We previously demonstrated that MilA, a CMP hydroxymethylase in the mildiomycin biosynthetic gene cluster in Streptomyces rimofaciens ZJU5119, can convert CMP to hmCMP12. MilA and CH are akin to the superfamily of thymidylate synthases (TS), which transfers a methyl group from CH2THF to dUMP to form dTMP in the de novo thymidylate synthesis pathway and, hence, DNA synthesis. In this study, we demonstrated that MilA has a substrate preference for CMP (kcat/KM = 39.2 mM−1 min−1) over dCMP (kcat/KM = 7.84 mM−1 min−1), and thus offers an opportunity to investigate the mechanism by which conserved TS evolves the preference for ribosyl over 2′-deoxyribosyl groups. In the structures of apo MilA and its complexes with various substrates, MilA are all homodimers.

The crystal structures of apo MilA, MilA in complexes with CMP, dCMP and hmCMP were determined. The structure of C-terminally His-tagged MilA was determined using selenomethionine (SeMet)-substituted MilA-L167M mutant at a 2.20 Å resolution. The electron density for residues 305–308 was poor in the structure of apo MilA but resolved clearly in the structures of all the MilA‒substrate complexes. There is no obvious difference between the structures of CMP-bound MilA and apo MilA, with the root-mean-square deviation (RMSD) being 0.34 Å for 634 aligned Cα atoms. The N-terminal three residues, C-terminal five residues, residue 232–238 of MilA, as well as the eight residues (LEHHHHHH) introduced by cloning, showed no clear electron density and presumably were disordered in the crystal. A MilA monomer consists of a six-stranded β-sheet, surrounded by thirteen α-helices and four 310-helices. Compared with TS and CH, MilA has an extra domain consisting of five α helices (from α9 to α13) in its C-terminal region. C-terminal truncations either from residue 235 or from residue 249 of MilA are both insoluble (data not shown). Presumably, this region could function as a domain to facilitate protein folding.

>METHTFGTFQDAYLSQLRDIYHSPEFRNAPRGQASRERIGAGFRLLDPVQRHISVPARRANVVFNFAEALWYLSGSDRLDFIQYYAPGIAAYSADGRTLRGTAYGPRIFRHPAGGVNQWENVVKTLTDDPDSKRAVIQIFDPRELAVADNIDVACTLALQFLIRDGLLCGIGYMRANDAFRGAVSDVFSFTFLQEFTARYLGLGIGTYHHVVGSVHIYDSDARWAERVLDAATPDGGPRPGFPAMPDGDNWPHVRRVLEWEERLRTNAARLSADALDALDLPAYWKHVVALFEAHRQVRHEDTPDRALLAALPEVYRQSLAVKWPGHFGSPAGSLEHHHHHH[2x]> TGGTHTPKLKHLDKLLAHCHRRRYTAKSTIIYAGDRCETLFFIIKGSVTILIEDDDGREMIIGYLNSGDFFGELGLFEKEGSEQERSAWVRAKVECEVAEISYAKFRELSQQDSEILYTLGSQMADRLRKTTRKVGDLAFLDVTGRVARTLLDLCQQPDAMTHPDGMQIKITRQEIGRIVGCSREMVG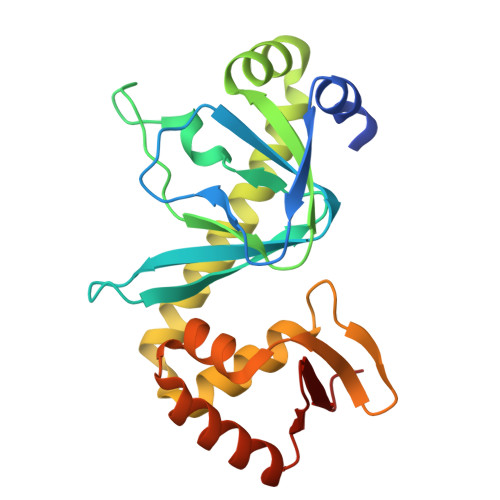RVLKSLEEQGLVHVKGKTMVVFGTR(2E)-3-{1-cyclopropyl-7-[(1S)-1-(3,6-dichloro-2-fluorophenyl)ethoxy]naphthalen-2-yl}prop-2-enoic acid | C24 H19 Cl2 F O3 | 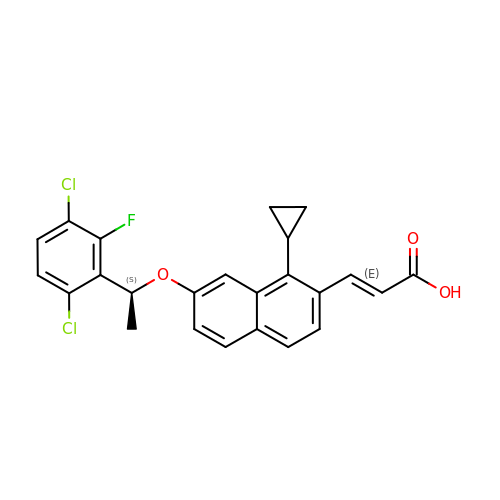JHFVJNXUDGWYLT-HJTPGIPUSA-N Recently, a selective thiosulfate uptake pathway involving a membrane protein YeeE (TsuA) in Escherichia coli was characterized. Here, we assessed selective thiosulfate transport via Spirochaeta thermophila YeeE in vitro and characterized E. coli YeeD (TsuB) as an adjacent and essential protein for YeeE-mediated thiosulfate uptake in vivo. YeeD is a cytoplasmic protein that belongs to the TusA (tRNA 2-thiouridine synthesizing protein A) protein family. Finally, the crystal structures of S. thermophila YeeE-YeeD fusion proteins at 3.34-Å and 2.60-Å resolutions revealed their interactions.

Introducing a mutation in YeeD (L45A) strengthened the interaction, as found in binding experiments using purified YeeE and YeeD mutants (described later). The mutants E15A, V16A, C17A, D42A, Y43A, E48A, and R49A severely impaired StYeeD’s affinity for StYeeE, while the mutant L45A enhanced the affinity. This enhanced affinity could stabilize the crystal packing of StYeeE-StYeeD, leading to its higher-resolution structure. Therefore, in this paper, we introduce Mol A of the higher resolution structure, which shows the best electron density map, to explain YeeE and YeeD interactions. The cytoplasmic indentation of StYeeE associates with StYeeD, which consists of 2 α-helices and 4 β-sheets. While the important, conserved residues C293, C91, and C22, termed the first, second, and third cysteines, respectively, are arranged perpendicular to the membrane at 8.6- and 6.7-Å intervals, C17 of StYeeD, one of the YeeE-interacting residues, is the putative enzymatic active site and is located adjacent to C22 of StYeeE as the “fourth cysteine. The distance between the third and the fourth cysteines, 10.8 Å, is wider than that between the other cysteines, and this space may be needed for transient binding of the thiosulfate ion rather than its transport. A water molecule is located at position III, a predicted thiosulfate-binding site. The relay of a thiosulfate ion from position III to C17 is likely facilitated by the conserved positively charged residues R28 and R98. In the 2.60-Å structure of StYeeE-StYeeD, the electron density is faint on the N-terminal side of the CPxP motif, raising the possibility that some electrons may be attracted to the CPxP motif.

>[2x]MIWTGLLVGFLFGIVLQRGRIAFNSAFRDVLLFKDNYLFKLAVFTLALEMILFVLLSQVGLMQMNPKPLNLVGNIIGGFVFGLGMVLAGGCASGVTYRVGEGLTTAWFAALFYGLGAYATKSGAFSWWLSWVGQFKSPLSVEESAYYVKGAGPTISSVLGLNPWIPALVIAALFILWAFGTKTTSRETKFNWKIASVCLALVAGLGFITSTLSGRKYGLGITGGWINLFQGFLTNSPLNWEGLEIVGIILGAGVAAAVAGEFKLRMPKNPVTYLQVGIGGLLMGIGAVTAGGCNIGHFLTGVPQLALSSWLASIFFILGNWTMAWILFRRAATPTPVAEAAPSSAEDRVLPFQVATGAVALQTAPRVKKAMANYQVSKEIDVRGEVCPIPDVEAKRAVQSANDGEIILVRIDYPASKERIPETVKKLGSEVLEIEEAAPGEWNIYIKVKKGSSGENLYFQ> MAHHHHHHVRPTVLCFSGLDPSGGAGLQADIEAIGQSGAHAAIACTALTIQNSQQVFGFEATSKELLLAQANAVVGDLPIKCVKSGMLGTTDNIAALAEFLRAHPDYQYVLDPVLVANSGGSLGDQATLV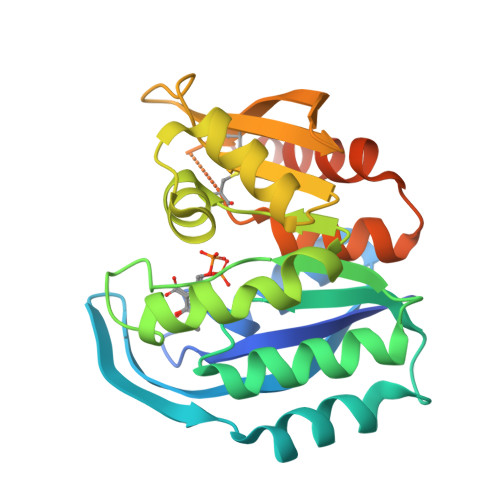KAFVELIPLATLITPNTVELRALTGVTDLDQATQKLFEMGAKAVLVKGGHEDTPDFIKNSLYIDGELAASSTCPRLEGEYHGSGCSLASFIAGRLALGDSLKIAVQHAETWLFGVLKNAETPVLNGQKIPKRF> MSLQLLRNTRIFVSTVKTGHDTTNTQEILVQDDISWGQDSNSTDITVNEAGPRPTRGSKRFNDSLNAAE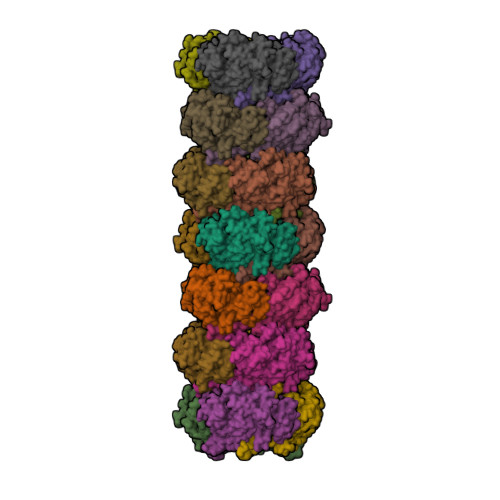WSFSTYILPYEDTTTGKQIVPDYMLWHALSSGKAIDLDGDTGAHNNATNFMVNFKDNAYHELAMLHIYILTDNAWSYIDSCQINQAEVNVDIEDIGRVTWSGNGNQLIPLDEQPFDPDALGIDDETYMTIQSSYIKNKLTILKIKDMDSDKEYDIPITGGTFTINNNITYLTPNIMSRVNIPIGSFTGAFELTGSLTAYLNDKSLGSMELYKDLVRTLKVVNRFEIALILGGEYDDERPAAVLVAKQAHVNIPTIETDDVLGTSVEFKAIPTDLDTGDEGYLGFSNKYTKTTVANLIATGDGAETPPILVESITVKSAADATSVTNSDTLQMSVEVTPPEATNTAVTWSISSGDAATIDAESGLLTADVSKTGEVIVKAVAKDGSGVEGTKTITVSAGE>[2x]PLIRVTLLEGRSPQEVAALGE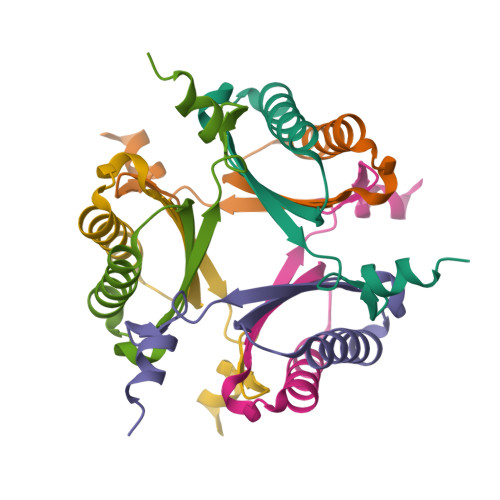ALTAAAHETLGTPVEAVRVIVEETPPERWFVGGRSVAERRASPS>[6x]SSPPVVDTVHGKVLGKFVSLEGFAQPVAIFLGIPFAKPPLGPLRFTPPQPAEPWSFVKNATSYPPMCTQDPKAGQLLSELFTNRKENIPLKLSEDCLYLNIYTPADLTKKNRLPVMVWIHGGGLMVGAASTYDGLALAAHENVVVVTIQYRLGIWGFFSTGDEHSRGNWGHLDQVAALRWVQDNIASFGGNPGSVTIFGESAGGESVSVLVLSPLAKNLFHRAISESGVALTSVLVKKGDVKPLAEQIAITAGCKTTTSAVMVHCLRQKTEEELLETTLKMKFLSLDLQGDPRESQPLLGTVIDGMLLLKTPEELQAERNFHTVPYMVGINKQEFGWLIPMLMSYPLSEGQLDQKTAMSLLWKSYPLVCIAKELIPEATEKYLGGTDDTVKKKDLFLDLIADVMFGVPSVIVARNHRDAGAPTYMYEFQYRPSFSSDMKPKTVIG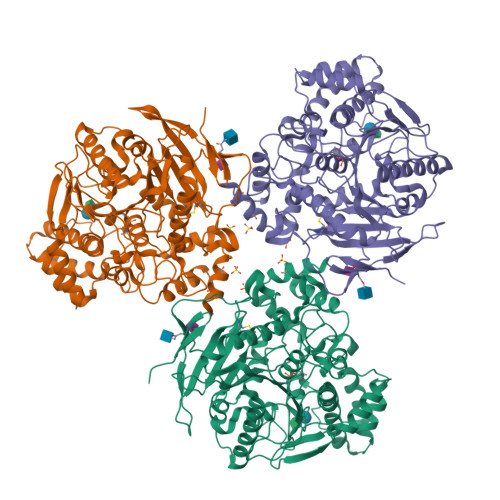DHGDELFSVFGAPFLKEGASEEEIRLSKMVMKFWANFARNGNPNGEGLPHWPEYNQKEGYLQIGANTQAAQKLKDKEVAFWTNLFAK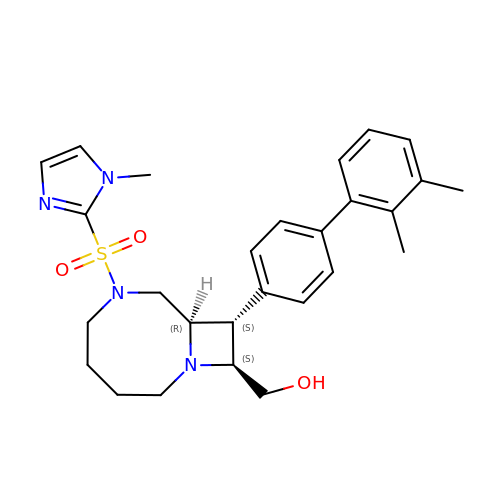{(8R,9S,10S)-9-(2',3'-dimethyl[1,1'-biphenyl]-4-yl)-6-[(1-methyl-1H-imidazol-2-yl)sulfonyl]-1,6-diazabicyclo[6.2.0]decan-10-yl}methanol | C27 H34 N4 O3 S | OJXBQVFJQWLDCX-NXCFDTQHSA-N>MGSHHHHHHMGQSVEVEILLNDAESRKRAEHKTEDGKKEKYFLFYDGETVSGKVSLSLKNPNKRLEHQGIKIEFIGQIELYYDRGNHHEFVSLVKDLARPGEITQSQAFDFEFTHVEKPYESYTGQNVKLRYFLRATISRRLNDVVKEMDIVVHTLSTYPELNSSIKMEVGIEDCLHIEFEYNKSKYHLKDVIVGKIYFLSVEIKIKHMEIDIIKRETTGTGPNVYHENDTIAKYEIMDGAPVRGESIPIRLFLAGYELTPTMRDINKKFSVRYYLNLVLIDEEERRYFKQQEVVLWRKGDIVRKSMSHQAAIASQRFEGTTS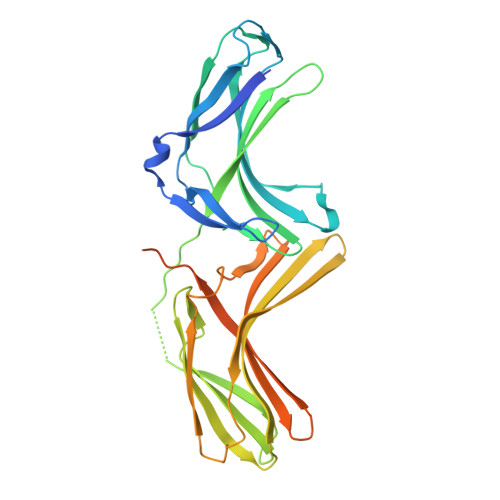LGEVRTPGQLSDNNSRQ[2x]> AT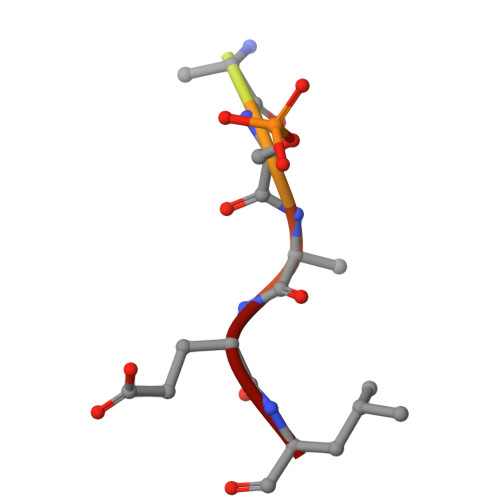KASQEL>[9x]MEDINFASLAPRHGTRPFMGTWNEIGTSQLNGGAFNWSSVWSGLKNFGSTLRTYGNKAWNSSTGQLLREKLKDQNFQQKVVDGLASGINGVVDIANQAVQREINSRLDPRPPTVVEMEDATLPPPKGEKRPRPDAEETILQVDEPPSYEEAVKAGMPTTRIIAPLATGVMKPATLDLPPPPAPAPPKATPVVQAPPVATAVRRVPARRQAQNWQSTLHSIVGLGVKSLKRRRCY;>MATPSMMPQWAYMHIAGQDASEYLSPGLVQFARATDTYFSLGNKFRNPTVAPTHDVTTDRSQRLTLRFVPVDREATTYLYKARFTLAVGDNRVLDMASTYFDIRGVLDRGPSFKPYSGTAYNSLAPKGAPNPSQWETKEKQGTTGGVQQEKDVTKTFGVAATGGINITNQGLLLGTDETAENGKKDIYADKTFQPEPQVGEENWQENEAFYGGRALKKDTKMKPCYGSFARPTNEKGGQAKFKPVNEGEQPKDLDIDFAYFDVPGGSPPAGGSGEEYKADIILYTENVNLETPDTHVVYKPGTSDNSSEINLVQQSMPNRPNYIGFRDNFVGLMYYNSTGNMGVLAGQASQLNAVVDLQDRNTELSYQLLLDSLGDRTRYFSMWNSAVDSYDPDVRIIENHGVEDELPNYCFPLNGTGTNSTYQGVKITNGNDGAEESEWEKDDAISRQNQICKGNVYAMEINLQANLWKSFLYSNVALYLPDSYKYTPANVKLPANTNTYEYMNGRVVAPSLVDAYINIGARWSLDPMDNVNPFNHPRNAGLRYRSMLLGNGRYVPFHIQVPQKFFAIKNLLLLPGSYTYEWNFRKDVNMILQSSLGNDLRVDGASVRFDSVNLYATFFPMAHNTASTLEAMLRNDTHDQSFNDYLSAANMLYPIPAKATNVPISIPSRNWAAFRGWSFTRLKTKETPSLGSGFDPYFVYSGSIPYLDGTFYLNHTFKKVSIMFDSSVSWPGND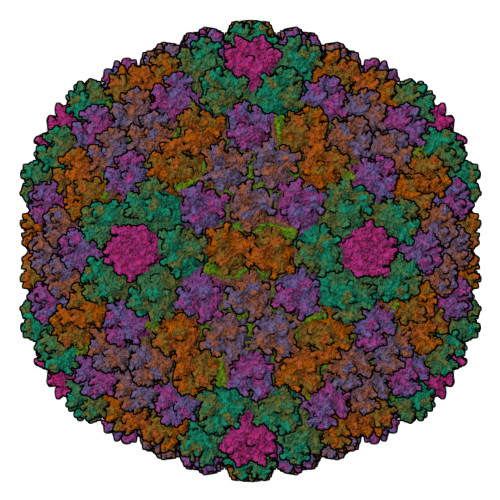RLLTPNEFEIKRSVDGEGYNVAQCNMTKDWFLVQMLSHYNIGYQGFHVPEGYKDRMYSFFRNFQPMSRQVVDEINYKDYKAVTLPFQHNNSGFTGYLAPTMRQGQPYPANFPYPLIGQTAVPSVTQKKFLCDRVMWRIPFSSNFMSMGALTDLGQNMLYANSAHALDMTFEVDPMDEPTLLYLLFEVFDVVRVHQPHRGVIEAVYLRTPFSAGNATT[12x];> MSQQAPDPAIRAALQSQPSGLASDDWEAAMQRIMALTTRNPESFRQQPQANRLSAILEAVVPSRTNPTHEKVLAIVNALAENKAIRPDEAGLVYNALLERVGRYNSTNVQSNLDRLVTDVREAVAQRERFKNEGLGSLVALNAFLATQPANVPRGQDDYTNFISALRLMVTEVPQSEVYQSGPDYFFQTSRQGLQTVNLSQAFKNLRGLWGVQAPVGDRSTVSSLLTPNSRLLLLLIAPFTDSGSVNRNSYLGHLLTLYREAIGQAQVDEQTFQEITSVSRALGQNDTDSLRATLNFLLTNRQQKIPAQYALSAEEERILRYVQQSVGLFLMQEGATPSAALDMTARNMEPSMYAANRPFINKLMDYLHRAAAMNTDYFTNAILNPHWLPPPGFYTGEYDMPDPNDGFLWDDVDSAVFSPTFQKRQEAPPSEGAVGRSPFPSLGSLHSLPGSVNSGRVSRPRLLGEDEYLNDSLLQPPRAKNAMANNGIESLVDKLNRWKTYAQDHRDAPAPRRQRHDRQRGLVWDDEDSADDSSVLDLGGSGGVNPFAHLQPKLGRRMF;> MRRAVVSSSPPPSYESVMAQATLEVPFVPPRYMAPTEGRNSIRYSELAPQYDTTRVYLVDNKSADIASLNYQNDHSNFLTTVVQNNDFTPAEASTQTINFDERSRWGGDLKTILHTNMPNVNEYMFTSKFKARVMVSRKHPEGVVETDLSQDKLEYEWFEFTLPEGNFSETMTIDLMNNAILENYLQVGRQNGVLESDIGVKFDSRNFKLGWDPVTKLVMPGVYTYEAFHPDVVLLPGCGVDFTESRLSNLLGIRKKQPFQEGFRIMYEDLEGGNIPALLDVPKYLESKKKVEDETKNAAAATADTTTRGDTFATPAQETAADKKVEVLPIEKDESGRSYNLIQGTHDTLYRSWYLSYTYGDPEKGVQSWTLLTTPDVTCGAEQVYWSLPDLMQDPVTFRSTQQVSNYPVVGAELMPFRAKSFYNDLAVYSQLIRSYTSLTHVFNRFPDNQILCRPPAPTITTVSENVPALTDHGTLPLRSSIRGVQRVTVTDARRRTCPYVYKALGIVAPRVLSSRTF;> MAKRLRVEDDFNPVYPYGYARNQNIPFLTPPFVSSDGFKNFPPGVLSLKLADPITINNGDVSLKVGGGLAVEQQTGNLSVNPDAPLQVASDKLQLALAPPFEVRDGKLALKAGNGLKVLDNSITGLTGLLNTLVVLTGRGIGTEELKNDDGVTNKGVGLRVRLGDDGGLTFDKKGDLVAWNKKDDRRTLWTTPDTSPNCKMSTEKDSKLTLTLTKCGSQVLGNVSLLAVTGEYHQMTATTKKDVKISLLFDENGILLPSSSLSKDYWNYRSDDSIVSQKYNNAVPFMPNLTAYPKPSAQNAKNYSRTKIISNVYLGALTYQPVIITIAFNQETENGCAYSITFTFTWQKDYSAQQFDVTSFTFSYLTQENKDKD;>MNGTGGAFEGGLFSPYLTTRLPGWAGVRQNVMGSTVDGRPVLPANSSTMTYATVGNSSLDSTAAAAAAAAAMTATRLASSYMPSSGSSPSVPSSIIAEEKLLALLAELEALSRQLAALTQQVSELREQQQQQNK[4x];>[2x]MSKEIPTPYMWSYQPQMGLAAGASQDYSTRMNWLSAGPSMISRVNGVRSHRNQILLEQAAVTSTPRAKLNPRNWPSTLVYQEIPGPTTVLLPRDALAEVRMTNSGVQLAGGASRCPLRPQSGIKTLVIRGRGTQLNDELVSSSIGLRPDGVFQLAGAGRSSFTPNQAYLTLQSSSSEPRSGGIGTLQFVEEFVPSVYFNPFSGSPGLYPDEFIPNFDAVREAVDGYD>QDAKAGEAVFKQCMTCHRADKNMVGPALAGVVGRKAGTAAGFTYSPLNHNSGEAGLVWTADNIVPYLADPNAFLKKFLTEKGKADQAVGVTKMTFKLANEQQRKDVVAYLATLK[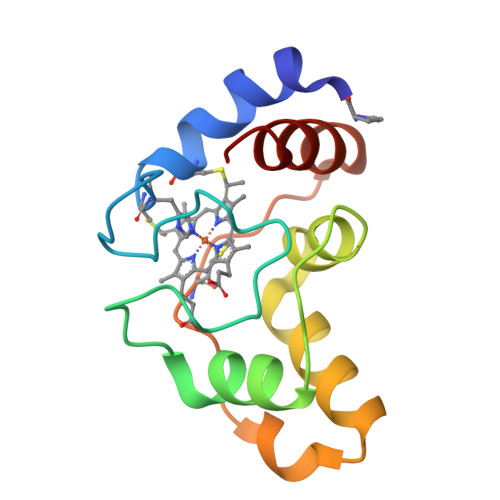4x]>MQLQELHMLVVLAEELNMRKAAERLFVSQPALSQRLQTIEKAWGTKIFLRSQKGL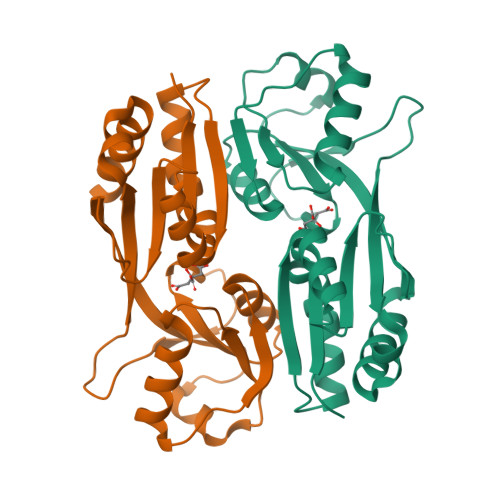TVTPAGEKIIQFANDVTDRQERIRENIDELEGEIHGTLKLAVASIIGQHWLPKVLKTYVERYPNAKVSLITGWSSEMLKSLYEDQVHIGIIRGNPEWKGRKDYLMTDHLYLVDTEISCIDDIAHTDRPFIQFKSDSTYFQEIQHWWHQKFKTSPKQTILVDQIETCKQMALHGIGYAILPSVTLEEEDKVNKMPLLDTKDHPIGRDTWLLGYEPAFELKQVQAFVSVIKDMLKQERPF[5x]>MAAQATAETPAGELPVIDAVTTHAPEVPPAIDRDYPAKVRVKMETVEKTMKMDDGVEYRYWTFDGDVPGRMIRVREGDTVEVEFSNNPSSTVPHNVDFHAATGQGGGAAATFTAPGRTSTFSFKALQPGLYIYHCAVAPVGMHIANGMYGLILVEPKEGLPKVDKEFYIVQGDFYTKGKKGAQGLQPFDMDKAVAEQPEYVVFNGHVGALTGDNALKAKAGETVRMYVGNGGPNLVSSFHVIGEIFDKVYVEGGKLI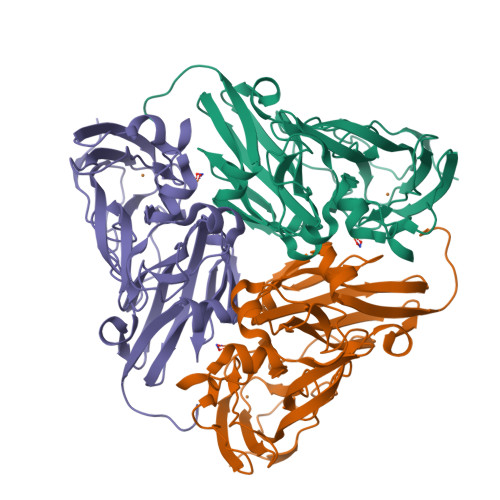NENVQSTIVPAGGSAIVEFKVDIPGNYTLVDHSIFRAFNKGALGQLKVEGAENPEIMTQKLSDTAYAVPR[6x]Feruloyl esterases (FAEs, E.C. 3.1.1.73), a subfamily of carboxylic acid esterases, are mainly associated with the release and exploitation of HCAs from plant cell walls. In this study, we aimed to obtain and characterize a feruloyl esterase (LaFae) from Lactobacillus acidophilus. To further investigate the active site configuration of LaFae, crystal structures of unliganded and ethyl ferulate-bound LaFae were determined at 2.3 and 2.19 Å resolutions, respectively. Seven α-helices surround the β-sheets and form a core domain that contains an active site with conserved catalytic triad residues (Ser106, Asp197 and His225).

The crystal of unliganded LaFae belongs to the space group of P212121 with two molecules in the asymmetric unit. The crystal structure of LaFae contains nine α helices and eight β strands. The β1 and β2 strands form an antiparallel β-sheet while the β3–β8 strands form parallel β-sheets. The α5- and α6-helices form a cap domain (from Ala133 to Val175). These structural features showed a canonical α/β fold of esterases. In the LaFae crystal structure, the α3, α4, α6 and α7 helices, as well as the β1-β2 hairpin, are involved in the dimerization interface. Several hydrogen bonds (Asp9-Leu11, Asp94-Lys86 and Leu118-Arg171) and salt bridges (Arg8-Asp9, Asp74-Lys86, Asp121-Arg171 and Asp121-His153) were observed at the dimerization interface; however, hydrophobic interactions (Ile81, Ala82, Leu118, Phe168, Val175, Leu176, Pro177 and Ile181) were predominant during the dimerization of LaFae. The substrate binding pocket is comprised of the β3-α1 loop, β7-α8 loop and β8-α9 loop regions. In addition, the cap domain was observed to be located above the ligand-binding site and this domain was hypothesized to have a gatekeeper role for substrate binding and release of the reaction product. Structural analysis shows that a Phe34 residue, located at the active site entrance, acts as a gatekeeper residue and controls substrate binding.

>SMSRITIERDGLTLVGDREEPFGEIYDMAILMHGFTANRNTPLLRQIADNLRDENVASVRFDFNGHGESDGAFEDMTVCNEIADAQKILEYVRTDPHVRNIFLVGHSQGGVVASMLAGLYPDIVKKVVLLAPAAQLKDDALNGDTQGATYNPEHIPAAIPFHGKKLGGFYLRTAQVLPIYEIAKHYTNPVSIIVGSNDQVVAPKYSKKYDEVYENSELHMVPDADHSFTGQYKDSAVDLTAEFLKPLF[2x]>MAPVLGYWKIRGLAQPIRLLLEYVGDSYEEHSYGRCDGEKWQNDKHNLGLELPNLPYYKDGNFSLTQSLAILRYIADKHNMIGNTPVERAKISMIEGGLVDLRAGVSRIAYQETFEQLKVPYLQQLPSTLRMWSQFLGNNSYLHGSTPTHLDFMFYEALDVIRYLDPTSVEAFPNLMQFIHRIEALPNIKA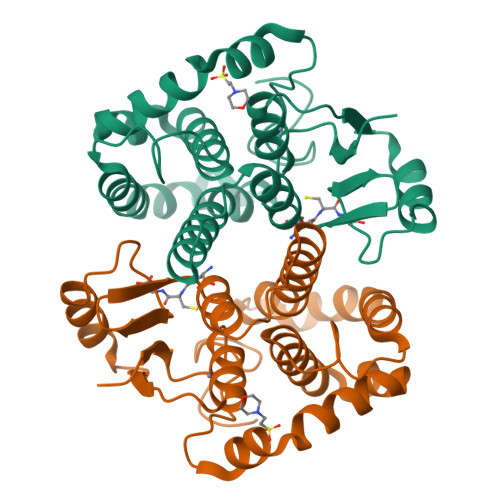FMESDRFIKWPLNGWSAYFGGGDAPPK[2x]1-[5-[4-(ethoxyiminomethyl)phenoxy]-3-methyl-pentyl]-3-pyridin-4-yl-imidazol-2-one | C23 H28 N4 O3 | 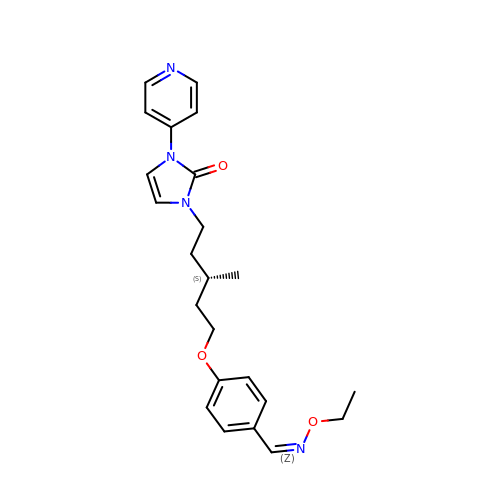JVWDSRHSJUZDAL-BWAHOGKJSA-N> MSAMKRPRSNSIVEETAVSAYVQTCTNFKSNVTFTDISKVSCVAYHVLLVGALEQLRDNSLKSVLFYCPAVAEALQRVKAGSTVKTLAEVPGRKGYTEVMVTALPATTSRTNCPYRADSMSEAVAAACGSVEEGEVLDVYVCAPAGSETAVANAVARAAPHSYTAKAGQATKAYMKQAMSLNVVMSSRAAFTQELVRGKSVCVAELEAICTSVQLCQRLVDTPPCMLDTVVYAEIAAAYAAELGVDMTVIKGDELREKGYGGIYAVGKCAQYPAHLVTLRYRNPNAAEGAKNIAMVGKGIVYDCG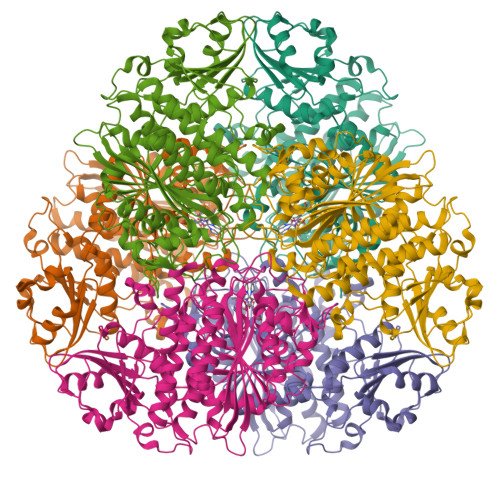GLALKPAAHMTNMKTDMGGSAGVFCAFIAVVRSMKMQRTHFSHIANISVTLCLAENAIGPHSYRNDDVVVMKSGKSVEVMNTDAEGRIVLGDGVYYATGEQDFVPDVLIDMATLTGAQGVATGSKHAGVYASDAEAEKDMISAGLQSGDLCYPVLYCPEYHEEVYKSPCADMRNIANSSSSAGSSCGGYFVEQHLSERFRGPFVHVDMAYPTSNTAGATGYGVTLVFEFLRQH> SDSAFANLDAAGFLQIWQHFDADDNGYIEGKELDDFFRHMLKKLQPKDKITDERVQQIKKSFMSAYDATFDGRLQIEELANMILPQEENFLLIFRREAPLDNSVEFMKIWRKYDADSSGYISAAELKNFLKDLFLQHKKKIP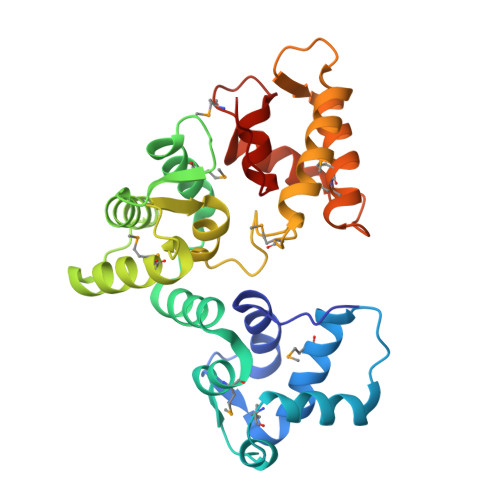PNKLDEYTDAMMKIFDKNKDGRLDLNDLARILALQENFLLQFKMDASSQVERKRDFEKIFAHYDVSRTGALEGPEVDGFVKDMMELVRPSISGGDLDKFRECLLTHCDMNKDGKIQKSELALCLGLKHKP> MEGKMFIGGLSWDTTKKDLKDYFSKFGEVVDCTLKLDPITGRSRGFGFVLFKESE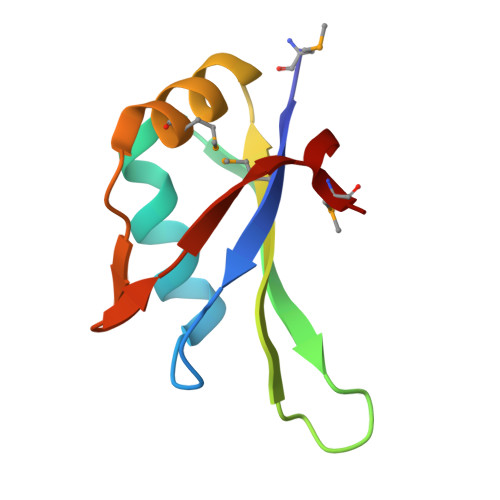SVDKVMDQKEHKLNGKVIDPKRAKAMA> CCACUGAGAGUUUC;> GGAAGCUCUGACCGACCCCCAGCC;> GCUGGGACAACUAGACA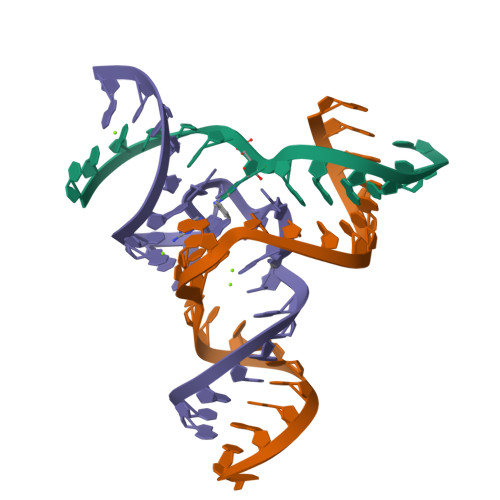UACAGUG>[2x]MKFNKVKLVIHACVLLFIIISIALIFHRLQTKTHSIDPIHKETKLSDNEKYLVDRNKEKVAP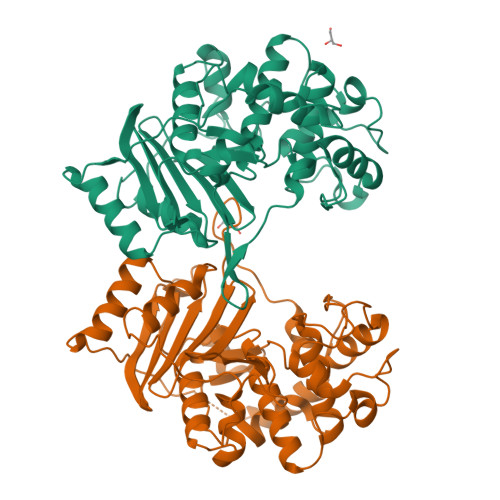SKLKEVYNSKDPKYKKIDKYLQSSLFNGSVAIYENGKLKMSKGYGYQDFEKGIKNTPNTMFLIGSAQKFSTGLLLKQLEEEHKININDPVSKYLPWFKTSKPIPLKDLMLHQSGLYKYKSSKDYKNLDQAVKAIQKRGIDPKKYKKHMYNDGNYLVLAKVIEEVTGKSYAENYYTKIGDPLKLQHTAFYDEQPFKKYLAKGYAYNSTGLSFLRPNILDQYYGAGNLYMTPTDMGKLITQIQQYKLFSPKITNPLLHEFGTKQYPDEYRYGFYAKPTLNRLNGGFFGQVFTVYYNDKYVVVLALNVKGNNEVRIKHIYNDILKQNKPYNTKGVIVQ> MYYPVSALLIEYLILAIVSKHDSYGYDISQTIKLIASIKESTLYPILKKLEKAGYLSTYTQEHQGRRRKYYHLTDSGEKHLVYLTKEWSVYKMTIDGIVEGRIRH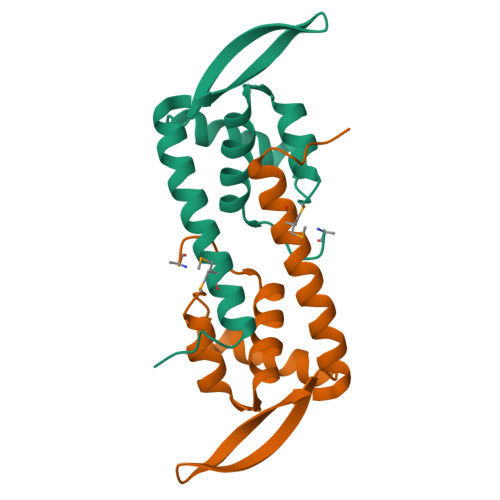DKN4,4,6,7,8,9-HEXAHYDROXY-5-METHYLCARBOXAMIDONONANOIC ACID | C11 H21 N O9 | 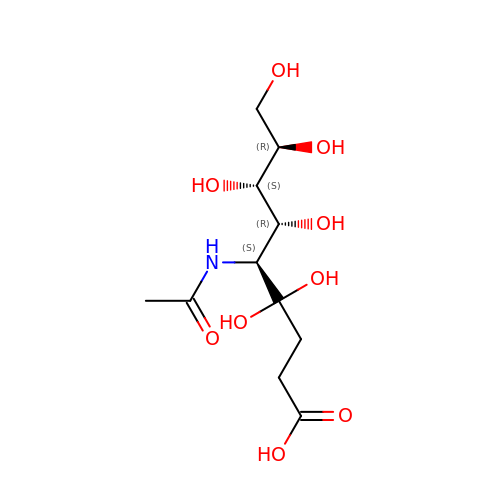LNLFFPBOMACCNX-PRQTWWFRSA-N>GAMEVEVKLRLLTAAAHLRLTTLLTPYHLKTLHQRNTFFDTPKNDLS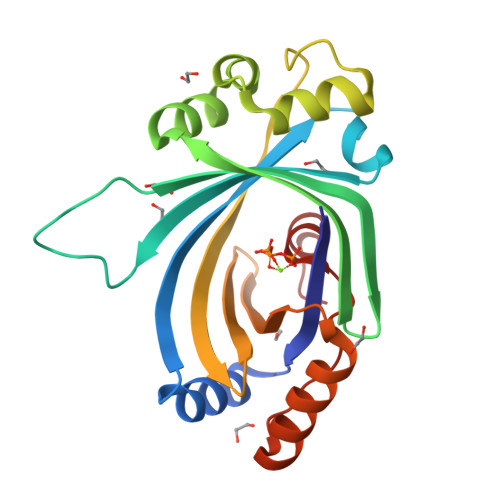LRRAVLRLRFLQNAAVSAASPSPPRCIVSLKAKPTLANGISRVEEDEEEIEYWIGKECVESPAKLSDIGSRVLKRVKEEYGFNDFLGFVCLGGFENVRNVYEWRGVKLEVDETKYDFGNCYEIECETEEPERVKTMIEEFLTEEKIEFSNSDMTKFAVFRSGKLP[2x]>MMVTVEEEVYEFLKKKAKEEGTSVPAVIRKILKEYFGIEDRTRDYKRQDLEGSYIIVNGKKYYRINCKLEKRNEILVKLE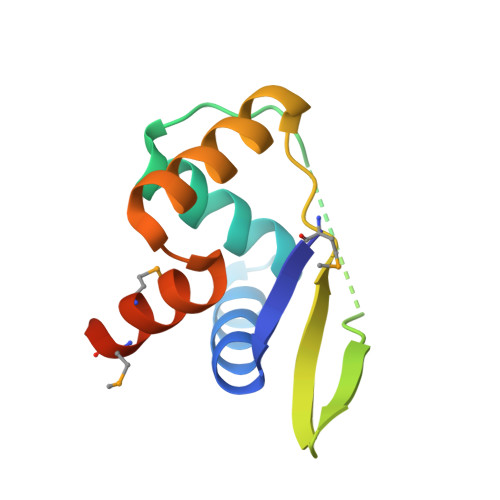LKKRGTTLNRFLKEMIMITVHHHHHH[4x]> MSLGAKPFGEKKFIEIKGRRMAYIDEGTGDPILFQHGNPTSSYLWRNIMPHCAGLGRLIACDLIGMGDSDKLDPSGPERYAYAEHRDYLDALWEALDLGDRVVLVVHDWGSALGFDWARRHRERVQGIAYMEAIAMPIEWADFPEQDRDLFQAFRSQAGEELVLQDNVFVEQVLPGLILRPLSEAEMAAYREPFLAAGEARRPTLSWPRQIPIAGTPADVVAIARDYAGWLSESPIPKLFINAEPGALTTGRMRDFCRTWPNQTE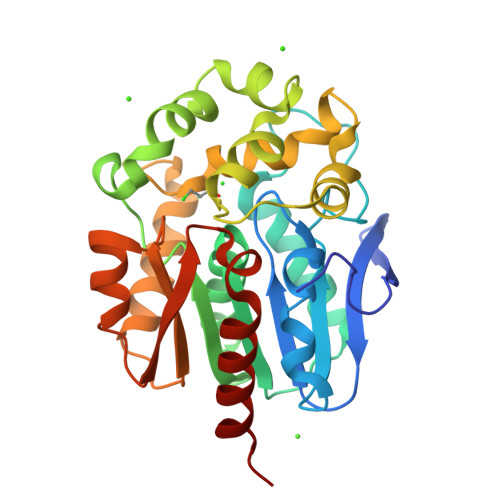ITVAGAHFIQEDSPDEIGAAIAAFVRRLRPA> MLQPVFTLKLRHKISPRMVAVGRYDGTHPCLAAATQAGKVFIHNPHSRSQHLGAPRVLQSPLESDVSLLNINQTVSCLTAGVLNPELGYDALLVGTQTNLLAYDVYNNSDLFYREVADGASAIVLGTLGDITSPLAIIGGNCALQGFNHEGNDLFWTVTGDNVHSLALCDFDGDGKKELLVGSEDFDIRVFKEDEIVAEMSETEIITSLCPMYGSRFGYALSNGTVGVYDKTARYWRIKSKNQAMSIHAFDLNSDGVCELITGWSNGKVDARSDRTGEVIFKDNFSSAIAGVVEGDYRMEGCQQLICCSVDGEIRGYLPGTAEMRGNLMDISVEQDLIRELSQKKQNLLLELRNYEENAKAELSSPLNEADGHRGVIPANTKHHTALSVSLGSEAQAAHAELCISTSNDTIIRAVLIFAEGVFAGE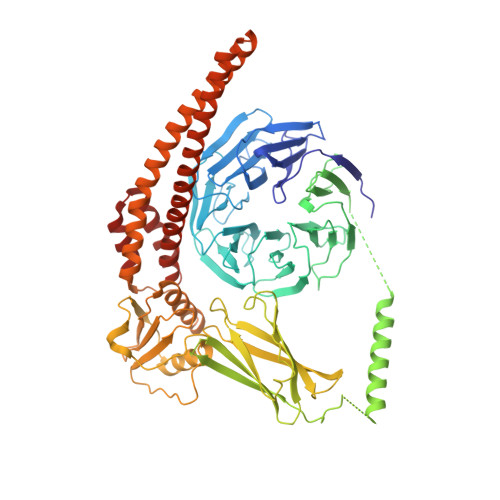SHVVHPSVHHLSSSVRIPITPPKDIPVDLHLKTFVGYRSSTQFHVFELTRQLPRFSMYALTSPDPASEPLSYVNFIIAERAQRVVMWLNQNFLLPEDTNIQNAPFQVCFTSLRNGGQLYIKIKLSGEITVNTDDIDLAGDIIQSMASFFAIEDLQVEADFPVYFEELRKVLVKVDEYHSVHQKLSADMADNSNLIRSLLVQAEDARLMRDMKTMKNRYKELYDLNKDLLNGYKIRCNNHTELLGSLKAVNQAIQRAGHLRVGKPKNQVITACRDAIRSNNINMLFRIMRVGTASS>[4x]GSTDNPDGIDYKTYDYVGVWGFSPLSNTNWFAAGSSTPGGITDWTATMNVNFDRIDNPSITVQHPVQVQVTSYNNNSYRVRFNPDGPIRDVTRGPILKQQLDWIRTQELSEGCDPGMTFTSEGFLTFETKDLSVIIYGNFKTRVTRKSDGKVIMENDEVGTASSGNKCRGLMFVDRLYGNAIASVNKNFRNDAVKQEGFYGAGEVNCKYQDTYILERTGIAMTNYNYDNLNYNQWDLRPPHHDGALNPDYYIPMYYAAPWLIVNGCAGTSEQYSYGWFMDNVSQSYMNTGDTTWNSGQEDLAYMGAQYGPFDQHFVYGAGGGMECVVTAFSLLQGKEFENQVLNKRSVMPPKYVFGFFQGVFGTSSLLRAHMPAGENNISVEEIVEGYQNNNFPFEGLAVDVDMQDNLRVFTTKGEFWTANRVGTGGDPNNRSVFEWAHDKGLVCQTNITCFLRNDNEGQDYEVNQTLRERQLYTKNDSLTGTDFGMTDDGPSDAYIGHLDYGGGVEC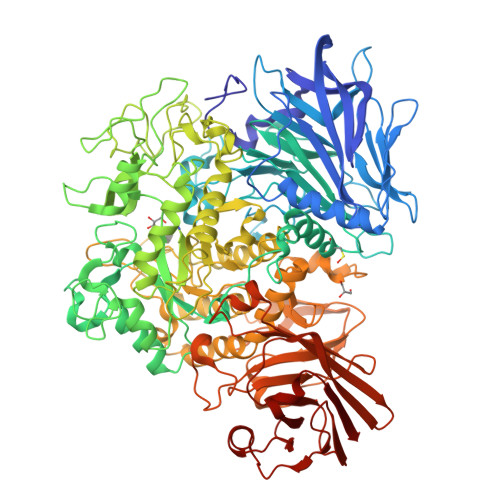DALFPDWGRPDVAEWWGNNYKKLFSIGLDFVWQDMTVPAMMPHKIGDDINVKPDGNWPNADDPSNGQYNWKTYHPQVLVTDMRYENHGREPMVTQRNIHAYTLCESTRKEGIVENADTLTKFRRSYIISRGGYIGNQHFGGMWVGDNSTTSNYIQMMIANNINMNMSCLPLVGSDIGGFTSYDNENQRTPCTGDLMVRYVQAGCLLPWFRNHYDRWIESKDHGKDYQELYMYPNEMDTLRKFVEFRYRWQEVLYTAMYQNAAFGKPIIKAASMYNNDSNVRRAQNDHFLLGGHDGYRILCAPVVWENSTERELYLPVLTQWYKFGPDFDTKPLEGAMNGGDRIYNYPVPQSESPIFVREGAILPTRYTLNGENKSLNTYTDEDPLVFEVFPLGNNRADGMCYLDDGGVTTNAEDNGKFSVVKVAAEQDGGTETITFTNDCYEYVFGGPFYVRVRGAQSPSNIHVSSGAGSQDMKVSSATSRAALFNDGENGDFWVDQETDSLWLKLPNVVLPDAVITIT>SVHHIKRRDIVLKWELGEGAFGKVFLAECHNLLPEQDKMLVAVKALKEASESARQDFQREAELLTMLQHQHIVRFFGVCTEGRPLLMVFEYMRHGDLNRFLRSHGPDAKLLAGGEDVAPGPLGLGQLLAVASQVAAGMVYLAGLHFVHRDLATRNCLVGQGLVVKIGDFGMSRDIYSTDYYRVGGRTMLPIRWMPPESILYRKFTTESDVWSFGVVLWEIFTYGKQPWYQLSNTEAIDCITQGRELERPRACPPEVY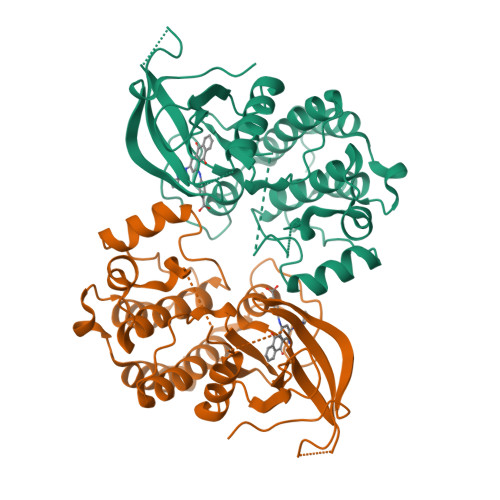AIMRGCWQREPQQRHSIKDVHARLQALAQAPPVYLDVLG[2x]>MAEYKDNLLGEANSFLEVLEQVSHLAPLDKPVLIIGERGTGKELIASRLHYLSSRWQGPFISLNCAALNENLLDSELFGHEAGAFTGAQKRHPGRFERADGGTLFLDELATAPMMVQEKLLRVIEYGELERVGGSQPLQVNVRLVCATNADLPAMVNEGTFRADLLDRLAFDVVQLPPLRERESDIMLMAEYFAIQMCREIKLPLFPGFTERARETLLNYRWPGNIRELKNVVERSVYRHGTSDYPLDDIIIDPFKRRPPEDAIAVSETTSLPTL[6x];>[2x]MQGSVTEFLKPRLVDIEQVSSTHAKVTLEPLERGFGHTLGNALRRILLSSMPGCAVTEVEIDGVLHEYSTKEGVQEDILEILLNLKGLAVRVQGKDEVILTLNKSGIGPVTAADITHDGDVEIVKPQHVICHLTDENASISMRIKVQRGRGYVPASTRIHSEEDERPIGRLLVDACYSPVERIAYNVEAARVEQRTDLDKLVIEMETNGTIDPEEAIRRAATILAEQLEAFVDLRDVRQPEVKEEKPEFDPILLRPVDDLELTVRSANCLKAEAIHYIGDLVQRTEVELLKTPNLGKKSLTEIKDVLASRGLSLGMRLENWPPASIADE;> MVYSYTEKKRIRKDFGKRPQVLDVPYLLSIQLDSFQKFIEQDPEGQYGLEAAFRSVFPIQSYSGNSELQYVSYRLGEPVFDVQECQIRGVTYSAPLRVKLRLVIYEREAPEGTVKDIKEQEVYMGEIPLMTDNGTFVINGTERVIVSQLHRSPGVFFDSDKGKTHSSGKVLYNARIIPYRGSWLDFEFDPKDNLFVRIDRRRKLPATIILRALNYTTEQILDLFFEKVIFEIRDNKLQMELVPERLRGETASFDIEANGKVYVEKGRRITARHIRQLEKDDVKLIEVPVEYIAGKVVAKDYIDESTGELICAANMELSLDLLAKLSQSGHKRIETLFTNDLDHGPYISETLRVDPTNDRLSALVEIYRMMRPGEPPTREAAESLFENLFFSEDRYDLSAVGRMKFNRSLLREEIEGSGILSKDDIIDVMKKLIDIRNGKGEVDDIDHLGNRRIRSVGEMAENQFRVGLVRVERAVKERLSLGDLDTLMPQDMINAKPISAAVKEFFGSSQLSQFMDQNNPLSEITHKRRISALGPGGLTRERAGFEVRDVHPTHYGRVCPIETPEGPNIGLINSLSVYAQTNEYGFLETPYRKVTDGVVTDEIHYLSAIEEGNYVIAQANSNLDEEGHFVEDLVTCRSKGESSLFSRDQVDYMDVSTQQVVSVGASLIPFLEHDDANRALMGANMQRQAVPTLRADKPLVGTGMERAVAVDSGVTAVAKRGGVVQYVDASRIVIKVNEDEMYPGEAGIDIYNLTKYTRSNQNTCINQMPCVSLGEPVERGDVLADGPSTDLGELALGQNMRVAFMPWNGYNFEDSILVSERVVQEDRFTTIHIQELACVSRDTKLGPEEITADIPNVGEAALSKLDESGIVYIGAEVTGGDILVGKVTPKGETQLTPEEKLLRAIFGEKASDVKDSSLRVPNGVSGTVIDVQVFTRDGVEKDKRALEIEEMQLKQAKKDLSEELQILEAGLFSRIRAVLVAGGVEAEKLDKLPRDRWLELGLTDEEKQNQLEQLAEQYDELKHEFEKKLEAKRRKITQGDDLAPGVLKIVKVYLAVKRRIQPGDKMAGRHGNKGVISKINPIEDMPYDENGTPVDIVLNPLGVPSRMNIGQILETHLGMAAKGIGDKINAMLKQQQEVAKLREFIQRAYDLGADVRQKVDLSTFSDEEVMRLAENLRKGMPIATPVFDGAKEAEIKELLKLGDLPTSGQIRLYDGRTGEQFERPVTVGYMYMLKLNHLVDDKMHARSTGSYSLVTQQPLGGKAQFGGQRFGEMEVWALEAYGAAYTLQEMLTVKSDDVNGRTKMYKNIVDGNHQMEPGMPESFNVLLKEIRSLGINIELEDE;> MKDLLKFLKAQTKTEEFDAIKIALASPDMIRSWSFGEVKKPETINYRTFKPERDGLFCARIFGPVKDYECLCGKYKRLKHRGVICEKCGVEVTQTKVRRERMGHIELASPTAHIWFLKSLPSRIGLLLDMPLRDIERVLYFESYVVIEGGMTNLERQQILTEEQYLDALEEFGDEFDAKMGAEAIQALLKSMDLEQECEQLREELNETNSETKRKKLTKRIKLLEAFVQSGNKPEWMILTVLPVLPPDLRPLVPLDGGRFATSDLNDLYRRVINRNNRLKRLLDLAAPDIIVRNEKRMLQEAVDALLDNGRRGRAITGSNKRPLKSLADMIKGKQGRFRQNLLGKRVDYSGRSVITVGPYLRLHQCGLPKKMALELFKPFIYGKLELRGLATTIKAAKKMVEREEAVVWDILDEVIREHPVLLNRAPTLHRLGIQAFEPVLIEGKAIQLHPLVCAAYNADFDGDQMAVHVPLTLEAQLEARALMMSTNNILSPANGEPIIVPSQDVVLGLYYMTRDCVNAKGEGMVLTGPKEAERLYRSGLASLHARVKVRITEYEKDANGELVAKTSLKDTTVGRAILWMIVPKGLPYSIVNQALGKKAISKMLNTCYRILGLKPTVIFADQIMYTGFAYAARSGASVGIDDMVIPEKKHEIISEAEAEVAEIQEQFQSGLVTAGERYNKVIDIWAAANDRVSKAMMDNLQTETVINRDGQEEKQVSFNSIYMMADSGARGSAAQIRQLAGMRGLMAKPDGSIIETPITANFREGLNVLQYFISTHGARKGLADTALKTANSGYLTRRLVDVAQDLVVTEDDCGTHEGIMMTPVIEGGDVKEPLRDRVLGRVTAEDVLKPGTADILVPRNTLLHEQWCDLLEENSVDAVKVRSVVSCDTDFGVCAHCYGRDLARGHIINKGEAIGVIAAQSIGEPGTQLTMRTFHIGGAASRAAAESSIQVKNKGSIKLSNVKSVVNSSGKLVITSRNTELKLIDEFGRTKESYKVPYGAVLAKGDGEQVAGGETVANWDPHTMPVITEVSGFVRFTDMIDGQTITRQTDELTGLSSLVVLDSAERTAGGKDLRPALKIVDAQGNDVLIPGTDMPAQYFLPGKAIVQLEDGVQISSGDTLARIPQESGGTKDITGGLPRVADLFEARRPKEPAILAEISGIVSFGKETKGKRRLVITPVDGSDPYEEMIPKWRQLNVFEGERVERGDVISDGPEAPHDILRLRGVHAVTRYIVNEVQDVYRLQGVKINDKHIEVIVRQMLRKATIVNAGSSDFLEGEQVEYSRVKIANRELEANGKVGATYSRDLLGITKASLATESFISAASFQETTRVLTEAAVAGKRDELRGLKENVIVGRLIPAGTGYAYHQDRMRRRAAG;> MARVTVQDAVEKIGNRFDLVLVAARRARQMQVGGKDPLVPEENDKTTVIALREIEEGLINNQILDVRERQEQQEQEAAELQAVTAIAEGRR;> MKQGLQLRLSQQLAMTPQLQQAIRLLQLSTLELQQELQQALESNPLLEQTDLHDEVEAKEVEDRESLDTVDALEQKEMPDELPLDASWDEIYTAGTPSGNGVDYQDDELPVYQGETTQTLQDYLMWQVELTPFTDTDRAIATSIVDAVDDTGYLTIQIEDIVDSIGDDEIGLEEVEAVLKRIQRFDPVGVAAKDLRDCLLIQLSQFAKETPWLEEARLIISDHLDLLANHDFRTLMRVTRLKEEVLKEAVNLIQSLDPRPGQSIQTSEPEYVIPDVLVRKVSGRWTVELNADSIPRLKINQQYAAMGNSARNDADGQFIRSNLQEARWLIKSLESRNDTLLRVSRCIVEQQQAFFEQGEEYMKPMVLADIAQAVEMHESTISRVTTQKYLHSPRGIFELKYFFSSHVNTEGGGEASSTAIRALVKKLIAAENPAKPLSDSKLTSMLSEQGIMVARRTVAKYRESLSIPPSNQRKQLV

Bacteria use sigma (σ) factors to recruit RNA polymerase (RNAP) to promoter regions of genes that need to be transcribed, with 60% bacteria containing at least one specialized σ factor, σ54, responsible for transcribing many stress response genes. The σ54-mediated transcription initiation requires specific AAA+ proteins (ATPases Associated with diverse cellular Activities) known as bacterial enhancer-binding proteins (bEBPs). DNA looping enables bEBP hexamers to engage and actively remodel the RNAP-σ54-DNA closed complex to convert it into an open complex. In this work we capture intermediate states of bEBPs in facilitating DNA opening and partial unfolding of σ54, and therefore link the ATPase activity to DNA opening and σ54 remodeling, which eventually lead to transcription activation.

To understand the structural basis and how DNA is stabilized in these complexes, we determined the structures of PspF1-275-RNAP-σ54-DNA containing mismatches between −11 and −8 [RPi(−11/−8)] and between −10 and −1 [RPi(−10/−1)]. Interestingly, DNA with a partially opened bubble between −11 and −8 did not support transcription, suggesting that this complex is unable to proceed further to an open complex. In the RPi(−11/−8), we observe multiple structural conformations, at varying degrees of tilt of PspF1-275 hexamer ring relative to RNAP-σ54 and varying degrees of RNAP clamp opening We also observe significant degrees of promoter DNA bending, demonstrating the wide degree of conformational flexibility in the complex. The DNA density downstream of −10 was generally poorly resolved, indicating that this region was highly flexible. However, one conformation has sufficiently high resolution to allow us to resolve the DNA. In these complexes, we observe a previously unreported interaction between PspF and σ54 RpoN domain. This interaction is only possible with the tilted ring conformation, suggesting this interaction contributes to the stabilization of this ring conformation in both RPi(−11/−8) and RPi(−10/−1), giving rise to the higher-resolution reconstruction of these conformations. Significantly, we observe the σ54 N terminus is further shifted along the PspF hexamer in RPi(−11/−8) and RPi(−10/−1) compared to that of RPi(−12/−11). This would thus support the mechanistic model in which we proposed that ATP hydrolysis and the conformational changes within the hexamer lead to translocation of the σ54 N terminus; and RPi(−11/−8) and RPi(−10/−1) are further along the transcription initiation pathway. Second, PspF1-275 hexamer ring tilts, as observed in RPi(−11/−8) and RPi(−10/−1) structures, altering interactions between PspF1-275 and DNA, which could contribute to or stabilize DNA melting.> SRQLWKWSGNPTQRRGMKGKARKLFYKAIVRGKETLRIGDCAVFLSAGRPNLPYIGRIESLWESWGSNMVVK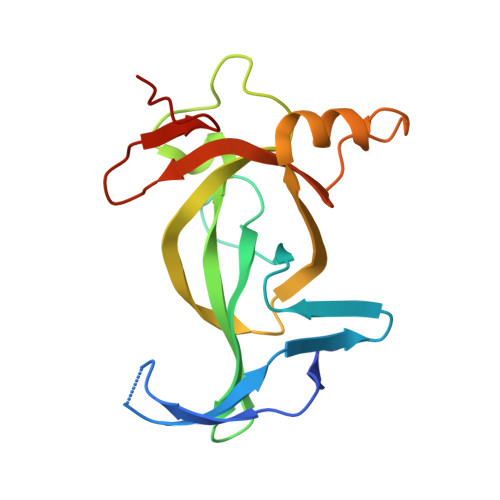VKWFYHPEETKLGKRQSDGKNALYQSCHEDENDVQTISHKCQVVGREQYEQMMRGRKYQDQQDLYYLAGTYDPTTGRLVTADGVPVLC>[2x]SNALQHTTIGDVLREHRRSHPGRTALVDGPVRLTWPELDDRVNRLAGSLAASGIGRGDRIMWLGQNSFRVYELIAAAGKLGAMVCVGYWRWAPPEMEFALRDFDPHLVVWQHQEIHETVARTREALGSDDTARWLRHDSAPQDPDGYEAFLAAGGLADPDLDIDPDSPVLVLYTAA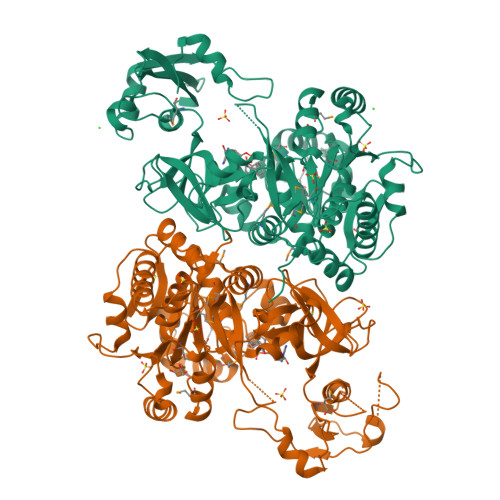MSGRQCGSLLSHTNLIAMATAAAWLGDIDHTTAFLNSGPMFHIGNHQFWGMPTLLMAGKNVIVRRVVAEEVRDLLVAEECTHAFLMPPTVAEIVRLNRDTGHDLSRLRATVAPHLWEGMATTDTSRFTRSGAAAGRGYGQTELSGFAVTAAYGGPAAGNAGRPGPGLTVRVLDTAGRECAVGEAGEICARGTVVHRGYWNRDEVNAHRFRSGWWHTTDLGRREPDGSLTFLGTTTRMLKSAAENIFPAEVENCIEQHPAVREAAVIGVPNTRWAQDVKAVVVLEPDAGVSEQEIIDHCRPRIASYKKPKSVAFAAALPRTVSGARDYDALDKEYGGGGYPGAATLGPGR1-~{tert}-butyl-3-[1-[(2~{S})-3-(3-carbamimidoylphenyl)-2-[[3-(3-carbamimidoylphenyl)phenyl]sulfonylamino]propanoyl]piperidin-4-yl]urea 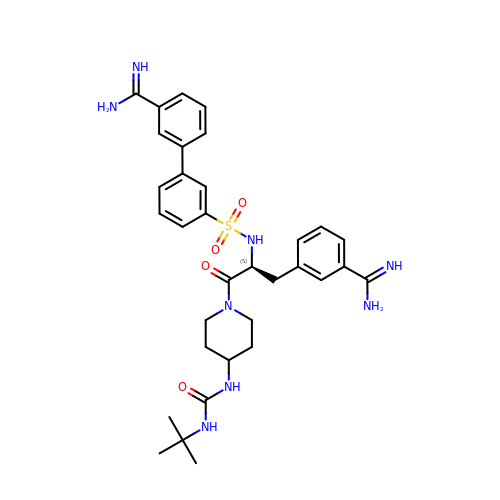| C33 H42 N8 O4 S | JFMRSUSVFPNDAU-NDEPHWFRSA-N>[2x]MAVSELEVDGVVFPSLARPPGSAHSHFLAGAGVRGMEIGGNFIKFTAIGVYLQADAAVSALAKKWAGKAADELASDAAFFRDVVTGEFEKFTQ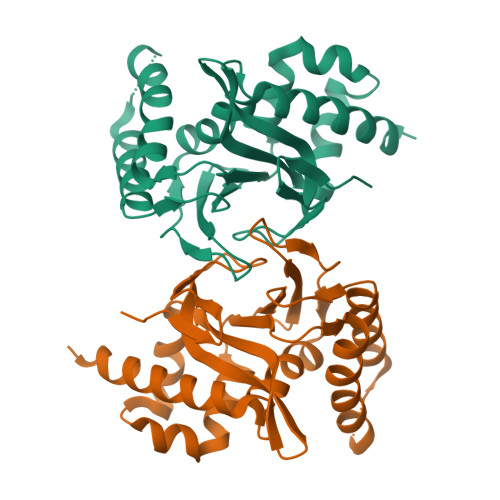VTMILPLTGAQYSEKVTENCVAYWKAVGAYTDAEAAAVDKFKEAFKTETFPPGASILFTHSPAGVLTVAFSKNSSVPESGGAAIENRPLCEAVLESIIGEHGVSPAAKLSLATRVAELLKEAASVDEPAAAEPVSVSA>MNTLELSARVLECGAMRHTPAGLPALELLLVHESEVVEAGHPRRVELTISAVALGDLALLLADTPLGTEMQVQGFLAPA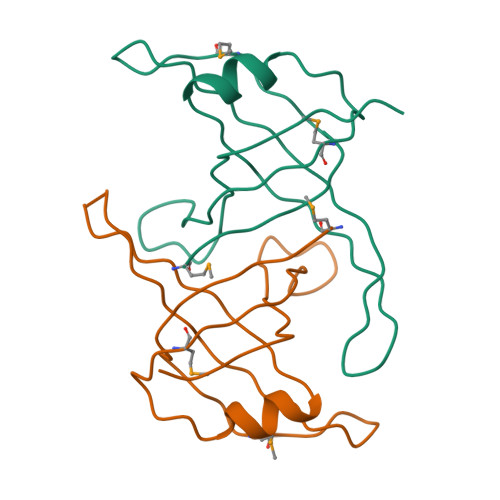RKDSVKVKLHLQQARRIAG[2x]[(2R,3S,5R)-5-(6-aminopurin-9-yl)-2-(phosphonooxymethyl)oxolan-3-yl] 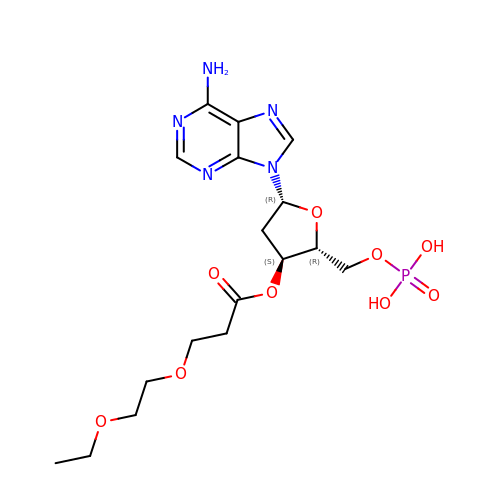3-(2-ethoxyethoxy)propanoate | C17 H26 N5 O9 P | YOZZSXDAZQISJN-YNEHKIRRSA-N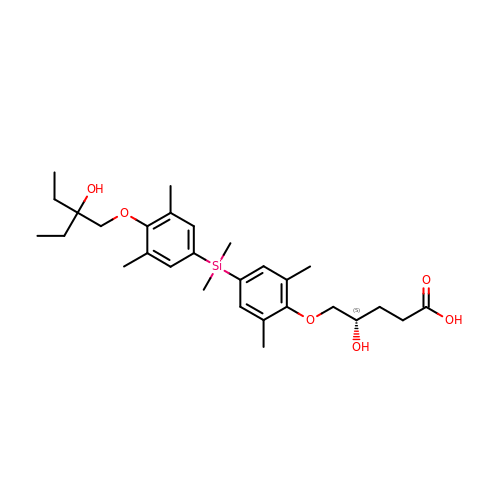(4~{S})-5-[4-[[4-(2-ethyl-2-oxidanyl-butoxy)-3,5-dimethyl-phenyl]-dimethyl-silyl]-2,6-dimethyl-phenoxy]-4-oxidanyl-pentanoic acid | C29 H44 O6 Si | NBCWQJGLMDGMMV-UHFFFAOYSA-N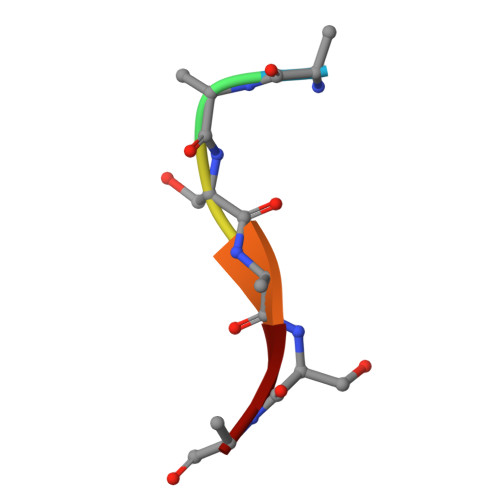> AASASA>GSHGGSEFELRRQASCLDNTSSVSGGDQTVCVTGAGGFIASWLVKLLLERGYTVRGTVRNPEDPKNG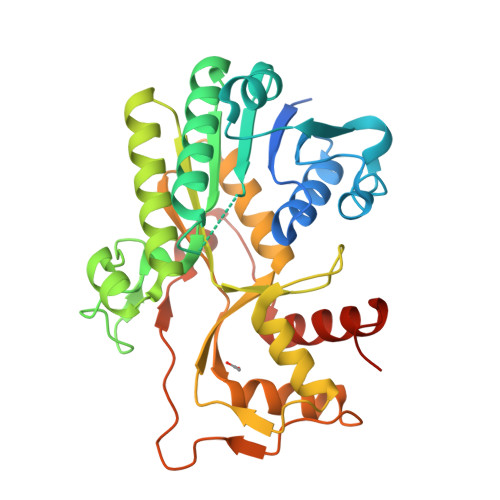HLKELEGARERLTLHKVDLLDLQSIQSVVHGCHGVFHTASPVTDNPDEMLEPAVNGTKNVIIASAEAKVRRVVFTSSIGTVYMDPNTSRDVVVDESYWSDLEHCKNTKNWYCYGKTVAEQSAWDIAKENQVDLVVVNPVVVLGPLLQPTINASTIHILKYLNGAAKTYVNATQSYVHVKDVALAHLLVYETNSASGRYICCETALHRGEVVEILAKYFPEYPLPTKCSDEKNPRVKPYKFSNQKLKDLGLEFTPVKQCLYDTVRSLQEKGHLPIPPMQEDSA[2x]> VESIIKTATDTVKSEINAELGVVPSLNAVETGATSNTEPEEAIQTRTV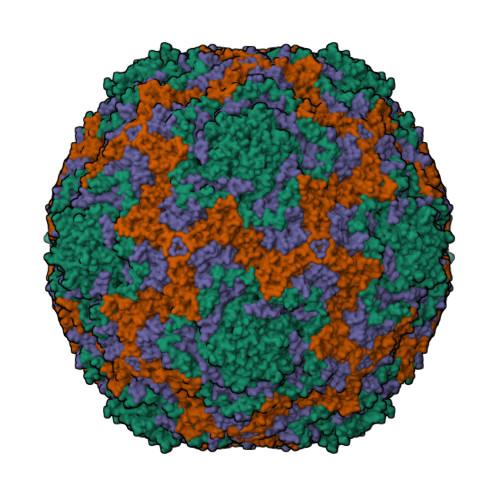INQHGVSETLVENFLGRAALVSKKSFEYKNHASSSAGTHKNFFKWTINTKSFVQLRRKLELFTYLRFDAEITILTTVAVNGNNDSTYMGLPDLTLQAMFVPTGALTPKEQDSFHWQSGSNASVFFKISDPPARMTIPFMCINSAYSVFYDGFAGFEKNGLYGINPADTIGNLCVRIVNEHQPVGFTVTVRVYMKPKHIKAWAPRPPRTMPYMSIANANYKGRDTAPNTLNAIIGNRASVTTMPHNIVTT;> SPSAEACGYSDRVLQLKLGNSAIVTQEAANYCCAYGEWPNYLPDHEAVAIDKPTQPETSTDRFYTLRSVKWESNSTGWWWKLPDALNNIGMFGQNVQYHYLYRSGFLIHVQCNATKFHQGALLVVAIPEHQRGAHDTTTSPGFNDIMKGERGGTFNHPYVLDDGTSIACATIFPHQWINLRTNNSATIVLPWMNVAPMDFPLRHNQWTLAVIPVVPLGTRTMSSVVPITVSIAPMCCEFNGLRHAITQ;> GVPTYLLPGSGQFLTTDDHSSAPVLPCFNPTPEMHIPGQIRNMLEMIQVESMMEINNTDGANGMERLRVDISVQADLDQLLFNIPLDIQLDGPLRNTLVGNISRYYTHWSGSLEMTFMFCGSFMATGKLILCYTPPGGSCPTTRETAMLGTHIVWDFGLQSSITLIIPWISGSHYRMFNSDAKSTNANVGYVTCFMQTNLIVPSESSDTCSLIGFIAAKDDFSLRLMRDSPDIGQSNHLHGAEAAYQ;> GAQVTRQQTGTHENANIATNGSHITYNQINFYKDSYAASASKQDFSQDPSKFTEPVVEGLKAGAPVLK Among the very few genes expressed during latency, the latency associated nuclear antigen 1 (kLANA) is the dominant protein expressed in all KSHV latently infected cells. LANA is required for the replication and maintenance of the viral episomes and thus is essential for latency. kLANA directs the replication and tethers the viral episome to mitotic chromosomes to ensure efficient segregation of the newly replicated molecules during mitosis. kLANA consists of 1162 amino acid residues divided into at least four unique regions, comprising a proline-rich region, a central acidic repeat region, a putative leucine zipper, and a dimerization and viral DNA binding domain (DBD). The distal C-terminus DBD is self-sufficient for both dimerization and DNA-binding. The DBD binds to specific sequences present within the terminal repeat (TR) of the viral episomal DNA, termed as LANA binding site (LBS).

Here we report the crystal structure of kLANA DBD forming a novel non-ring structure in the crystal packing. The structure was resolved at 3.8 Å resolution in space group C2221. The kLANA DBD structure determined consists of amino acid residues 1019–1150 with an additional two amino acid residues glycine and proline at the N-terminus resulting from the 3C protease tag cleavage. The asymmetric unit consists of four dimer molecules. The central two anti-parallel β-sheets of two monomers form a β-barrel dimer by burying several hydrophobic residues with an average buried surface area of 1123 Å2 per monomer. The three helices α1, α2 and α3 from each monomer flank the core β-barrel structure, α1 and α3 is involved in the higher oligomerization (see below) and α2 is proposed to interact with the DNA major groove. The tetramer interface forms a bend angle of about 102° between the two dimer molecules and is related by a crystallographic two fold axis. A similar interface has been reported previously but the angle between the dimer–dimer interfaces are 96° and 74° (the corresponding reported bend angles were 90° and 72° (27)) forming octameric and decameric ring structure, respectively. In addition to the bend angles, a greater rotational angle between dimers has been observed in the present structure, indicating more flexibility at this interface than previously known. With respect to the non-ring crystal structure, the relative rotation angles were 26° (octamer) and 14° (spiral). This ability to rotate may facilitate kLANA's cooperative binding and bending of DNA.

>GPVPYRQIDDCPAKARPQHIFYRRFLGKDGRRDPKCQWKFAVIFWGNDPYGLKKLSQAFQFGGVKAGPVSCLPHPGPDQSPITYCVYVYCQNKDTSKKVQMARLAWEASHPLAGNLQSSIVKFKKPLPLTQPGE[8x]N-(3-cyanophenyl)-2-methylpropanamide 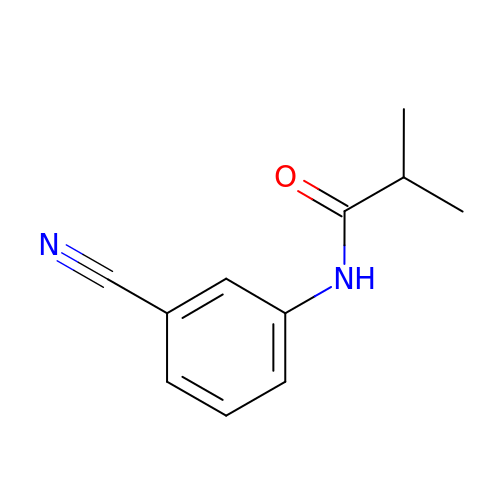| C11 H12 N2 O | JWBISRKEEZGPFB-UHFFFAOYSA-N In particular, RORγt, whose activity is required for the proliferation and functionality of immune Th17 cells, is the subject of intense investigation to modulate its activity to achieve clinical benefit. NRs are characterized by the ability to bind small ligands at a highly conserved hydrophobic orthosteric-binding pocket located within the protein's ligand-binding domain (LBD). Helix 12 (H12, also called activation function-2, AF-2) can adopt distinct conformations in response to ligand binding, regulating the interaction of the LBD with cofactor proteins with resulting changes in gene transcription at a particular locus. Here we characterize the mode of action of these inhibitors to guide an optimization program and surprisingly find a novel binding mode, thereby identifying the first allosteric-binding pocket for a highly potent, cellular active small NR ligand.

To elucidate the molecular basis of RORγt modulation by MRL-871, we performed co-crystallization studies with an equimolar complex of RORγt-LBD and MRL-871. Co-crystals grew in two different space groups. Crystals in space group R32:H had unit cell dimensions of a=b=173.8, c=67.2 Å, diffracted to 2.3 Å resolution and contain one molecule per asymmetric unit. The overall structures from both sets were identical in all the features and the ligand conformation. MRL-871 binds instead to a previously unidentified allosteric pocket in the RORγt LBD, located distal to the classical binding site (orange). Crystal structure analysis shows that this allosteric pocket, absent in the classical NR-folding motif, is formed by helices 4, 5, 11 and the reoriented flexible H12. The ortho-substituted trifluoromethyl and chloro moieties are spatially clearly positioned and impart a specific rotation to the phenyl group of MRL-871 and address hydrophobic sites in the allosteric pocket. Hydrogen-bonding interactions exist between the molecule's carboxylic acid group and the side chain of RORγt residue Q329 as well as the main-chain amide hydrogen atoms of residues A497 and F498. The arrangement of the RORγt LBD in the presence of MRL-871 generates a druggable molecular-binding site critically regulated by favourable interactions of MRL-871 with the AF-2 domain. These interactions reposition the highly flexible H12 in a conformation unique among reported NR ligand structures, of either the agonist or antagonist type, and distinct from the previously reported RORγt agonist-bound state. The unique conformation induced by the binding of MRL-871 prevents interaction with cofactor peptides, which typically bind RORγt through a conserved LXXLL motif, at the AF-2.

> ASLTEIEHLVQSVCKSYRETCQLRLEDLLRQRSNIFSREEVTGYQRKSMWEMWERCAHHLTEAIQYVVEFAKRLSGFMELCQNDQIVLLKAGAMEVVLVRMCRAYNADNRTVFFEGKYGGMELFRALGCSELISSIFDFSHSLSALHFSEDEIALYTALVLINAHRPGLQEKRKVEQLQYNLELAFHHHLCKTHRQSILAKLPPKGKLRSLCSQHVERLQIFQHLHPIVVQAAFPPLYKELFS>[4x]GSHMSASAEPESDVKGRILDAAADAFMLRGFANTTIDDIADDVGATKGLIYYHFRSKFDIFLAVYEDGMRRVRERVEPYVGAPGTGRQRLVAMSVAHVENLMIDLGYHHVVHQGVRDQAST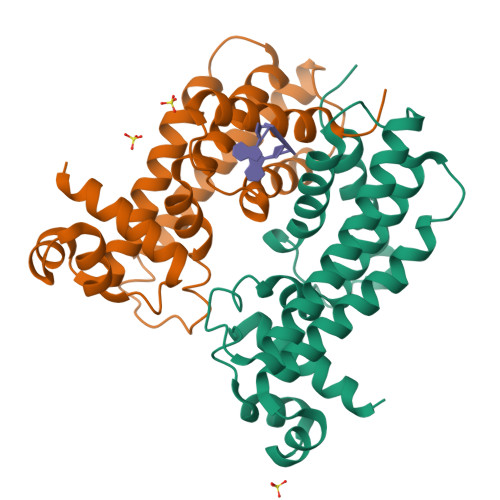ALKVRQRDALAALNELRRDYERMFHHVITEGIADGSLRNVDDALATRTLLSNLNAVDVWYRKIEGQTEKEVHDLASQVVDLLIGGIGATAD> GLPTMNTPGSNQFLTSDDFQSPCALPNFDVTPPIHIPGEVKNMMELAEIDT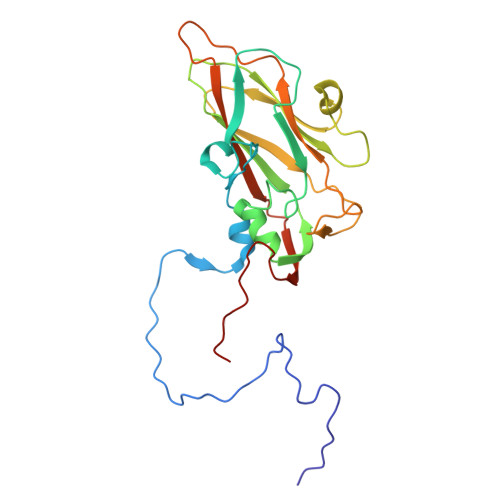LIPMNAVDGKVNTMEMYQIPLNDNLSKAPIFCLSLSPASDKRLSHTMLGEILNYYTHWTGSIRFTFLFCGSMMATGKLLLSYSPPGAKPPTNRKDAMLGTHIIWDLGLQSSCSMVAPWISNTVYRRCARDDFTEGGFITCFYQTRIVVPASTPTSMFMLGFVSACPDFSVRLLKDTPHISQSKLIGRTQ FKRP recognizes RboP-(phospho-)core M3 as the RboP acceptor and transfers a RboP from CDP-Rbo to form the tandem RboP structure. Although FKRP exhibits RboP transferase, not NTase activity, our crystal structure clearly shows that FKRP belongs to the NTase superfamily as proposed previously. Our structural and biochemical analyses revealed the acceptor substrate recognition mechanism by dimer FKRP: the phosphate group of RboP is recognized by the catalytic domain of one subunit, and a phosphate group on O-mannose is recognized by the stem domain of another subunit. Indeed, mutations of FKRP, which is involved in synthesis of a tandem RboP structure, cause congenital muscular dystrophy;17–23 more than 15 missense mutations in the FKRP gene were found in LGMD2I (limb-girdle muscular dystrophy type 2I), MDDGB5 [muscular dystrophy-dystroglycanopathy (congenital with or without mental retardation, type B, 5)], and severe muscle-eye-brain disease/Walker-Warburg syndrome (MEB/WWS) patients (OMIM ID of FKRP; 606596).

To understand the molecular basis of the unique substrate recognition and catalytic reaction of FKRP, we determined the crystal structures of the sFKRP-CDP-Rbo complex with Ba2+ and the sFKRP-CMP complex with Mg2+ at 2.23 Å and 2.60 Å resolution, respectively. Since the enzymatic activity does not appear in the presence of Ba2+, the whole substrate remained under the Ba2+-containing condition. In the CDP-Rbo complex structure, the α phosphate residue of CDP-Rbo seems to interact with the Ba2+ ion in site I. The loop region from Leu433 to Gln437, which is visible only in the CDP-Rbo complex structure, is involved in the interaction with the Rbo moiety (left gray loop). The CDP-Rbo complex structure suggests that the metal ion at site II, which could not be observed in the crystal structure, also interacts with the donor molecule CDP-Rbo. Upon CDP-Rbo binding, significant conformational changes of FKRP were induced in three regions: the zinc finger loop (Gly288 to Cys318), the Rbo-interacting loop (Leu433 to Gln437), and a C-terminal fragment (Pro481 to C-terminus). The most significant structural change occurred in the C-terminal fragment of subunits A and C. Upon CDP-Rbo binding, the α helix is unfolded and Gln482 makes an interaction with the CDP moiety of the CDP-Rbo. Moreover, a small hydrophobic patch was formed in the C-terminal fragment by Tyr483, Pro484, and Leu488 interacting with Asp303, Leu308, Tyr309, and Trp313 in the zinc finger loop by hydrophobic interaction and a hydrogen bond. These interactions shift the zinc finger loop toward the CDP moiety of CDP-Rbo; the shift was especially large around the residues Gly298 to Pro305. The hydrogen bond between Gln437 and CDP-Rbo seems to further stabilize the Rbo-interacting loop, covering the bound CDP-Rbo.

>GGRPAGPRVTVLVREFEAFDNAVPELVDSFLQQDPAQPVVVAADTLPYPPLALPRIPNVRLALLQPALDRPAAASRPETYVATEFVALVPDGARAEAPGLLERMVEALRAGSARLVAAPVATANPARCLALNVSLREWTARYGAAPAAPRCDALDGDAVVLLRARDLFNLSAPLARPVGTSLFLQTALRGWAVQLLDLTFAAARQPPLATAHARWKAEREGRARRAALLRALGIRLVSWEGGRLEWFGCNKETTRCFGTVVGDTPAYLYEERWTPPCCLRALRETARYVVGVLEAAGVRYWLEGGSLLGAARHGDIIPWDYDVDLGIYLEDVGNCEQLRGAEAGSVVDERGFVWEKAVEGDFFRVQYSESNHLHVDLWPFYPRNGVMTKDTWLDHRQDVEFPEHFLQPLVPLPFAGFVAQAPNNYRRFLELKFGPGVIENPQYPNPALLSLTGSG[4x]> MTAAVTPSASAVASDDKKSERRLAFWLIAPAVLLMLAVTAYPIGYAVWLSLQRYNLAEPHDTEFIGLANYVTVLTDGYWWTAFAVTLGITVVSVAIEFALGLALALVMHRTIFGKGAVRTAILIPYGIVTVAASYSWYYAWTPGTGYLANLLPEGSAPLTDQLPSLAIVVLAEVWKTTPFMALLLLAGLALVPQDLLNAAQVDGAGPWKRLTKVILPMIKPAILVALLFRTLDAFRIFDNIYILTGGSNDTGSVSILGYDNLFKAFNVGLGSAISVLIFLSVAIIAFIY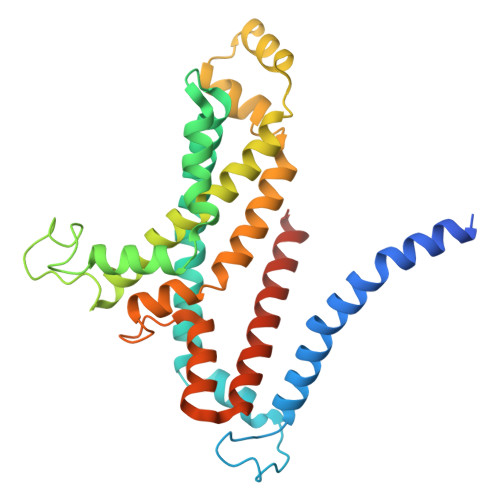IKIFGAAAPGSDEEVR> GSSHHHHHHSSGLVPRGSLTHRKFGGSGGSPFSGLSSIAVRSGSYLDAIIIDGVHHGGSGGNLSPTFTFGSGEYISNMTIRSGDYIDNISFETNMGRRFGPYGGSGGS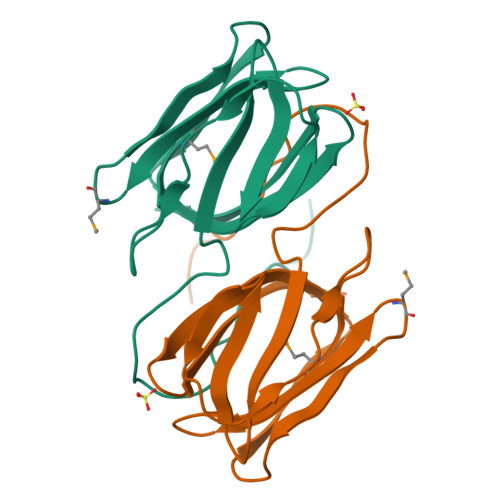ANTLSNVKVIQINGSAGDYLDSLDIYYEQY>GSAAPESLSPGATAEEAPEEDEDDAEAEDPERGTGSGGRSGSLGGSGGGTAGPGMALGGALTRRAVTLRVLLKDELLEPGEGVLSIYYLGRKFTGDLQLDGRIVWQETGQVFNSPSAWATHCKKLVNPAKKSGCGWASVKYKGQKLDKYKAAWLRRHQLHM[2x]

Recent research has identified the Mpr1/Pad1 N-terminal (MPN) domain-containing protein (MPND) as a sensor protein that may recognize DNA 6mA modification in eukaryotes. Moreover, the Mpr1/Pad1 N-terminal (MPN) domain-containing protein (MPND) was the first reported protein containing the RAMA domain to directly bind to DNA with the 6mA modification in vitro. In this work, we investigated the first crystal structures of the apo–MPND and the MPND–DNA complex from Mus musculus at the atomic resolution. Our results revealed that MPND possesses multiple functions, such as binding DNA and interacting with histones.

After extensive crystallization trials and optimizations, we successfully obtained MPND (residues 2–160) crystals suitable for diffraction experiments. The final apo–MPND structure in the space group P212121 was refined to 2.06 Å resolution, with an Rwork of 23.0% and an Rfree of 24.9%. In the final structural model, the asymmetric unit contained two protein protomers, each with three helices (α1–α3), two long antiparallel β-strands (β1–β2), and four short β-strands (β3–β6). Each protomer included MPND residues 62–156 with missing residues (131–133). According to the SDS-PAGE of crystals, the key reason the N-terminal structure could not be resolved was due to the conformational flexibility during crystallization rather than due to protein degradation. The two protomers possessed virtually identical spatial arrangements, as revealed by structural superposition, with an overall root-mean-square deviation (RMSD) of 1.0 Å for all Cα atoms. The main structural differences between the two protein protomers were in the irregular loops, particularly in the N-terminal location. Two MPND molecules were present in the asymmetric unit of the apo–MPND structure, but their interaction was weak. Interestingly, the structural analysis suggested two possible dimer configurations: dimer 1, which possessed an interface area of 439 Å2; and dimer 2, which was generated from the symmetry and possessed an interface area of 411 Å2. Therefore, the oligomeric state of apo–MPND in the solution is mainly monomeric.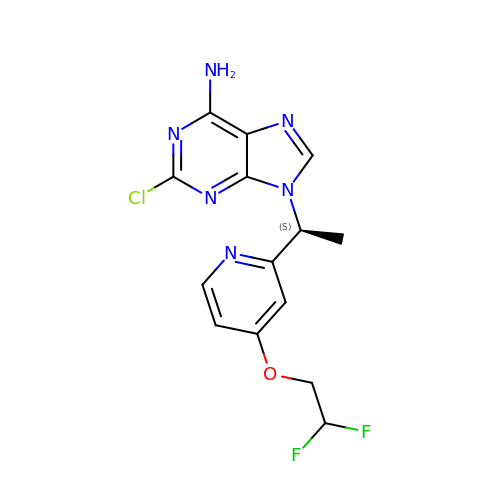9-[(1~{S})-1-[4-[2,2-bis(fluoranyl)ethoxy]pyridin-2-yl]ethyl]-2-chloranyl-purin-6-amine | C14 H13 Cl F2 N6 O | MMMUNMQNRGXDNZ-ZETCQYMHSA-N>[2x]MAFNPAPKAVQENHHVDYVIRFNYGDIDTPEAIKKFEVLLLELSEVGLQTEVRQGDENSLFVFVRAASKKKLKRAVYQSRVRDWLYGVRNTEPEPASSAKPQSEAERLLVIYHLITVPKAEGGAGITPRHGEWKNVDAIFPLHDEETNRQCMREWSKKTFLSTEDLDRIRNTFGEHVGFYFAFLQSYFRFLMFPAAFGFSCWLLLGSFSIIYTVVNCLWCIVFIEYWKRQEEDLSCRWQTKGVSAVHEKRAEFKPEKEIRDESTGEVRGVFPATKRMYRQLLQVPFALLAAVALGAIIATCFAIEIFISEVYNGPLKGYLVFIP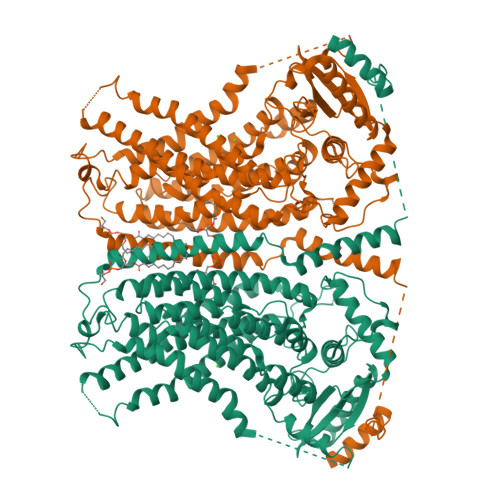TILVSALIPTMSAVLLTVATKLNDYENYETQDAYKVALTQKIFVVNFITSYLPIILTAFVYVPFASRIVPYLDVFHLTVRPFVSKEHAIKARTEFSINPDRLRKQVIYFTVTAQIVGFALETIVPFVKQRVFREYKEYTKKQHAKAEPGNGAGEKKTVSLGDDEDEARFLTRVRNEAELEDYDVTDDLREMCIQFGYLALFSPVWPLVPVSFLINNWVELRSDFFKICVECKRPWPQRADTIGPWLDSLGFLSWVGSITSSALVYMFSNGHEGPNGEPTTIRCWALLLTIFFSEHLYLIVRYAVRSALAKLEPPNTRRERIERFMMRKRYLDTVLSAESDDDADEVKGVVSSIPPSEITRESLEQDARDWSKQGTDPTERFWMRQRGWKESAEVGLSLITKAKGDETKKQQ> PEGLEQLEAQTNFTKRELQVLYRGFKNECPSGVVNEDTFKQIYAQFFPHGDASTYAHYLFNAFDTTQTGSVKFEDFVTALSILLRGTVHEKLRWTFNL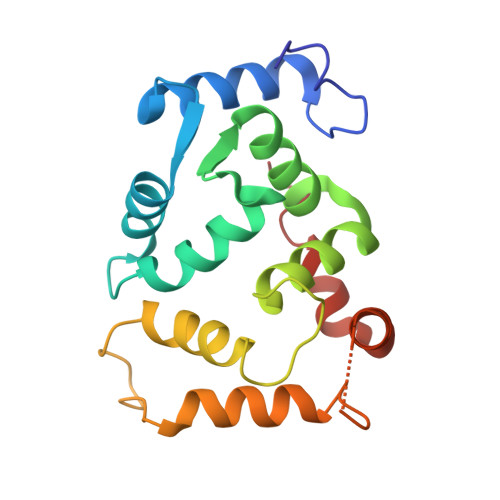YDINKDGYINKEEMMDIVKAIYDMMGKYTYPVLKEDTPRQHVDVFFQKMDKNKDGIVTLDEFLESCQEDDNIMRSLQLFQNVM methyl ~{N}-[4-[1-[(1~{R})-1-[5-[5-chloranyl-2-(1,2,3,4-tetrazol-1-yl)phenyl]-1-oxidanyl-pyridin-2-yl]-2-cyclopropyl-ethyl]pyrazol-4-yl]phenyl]carbamate 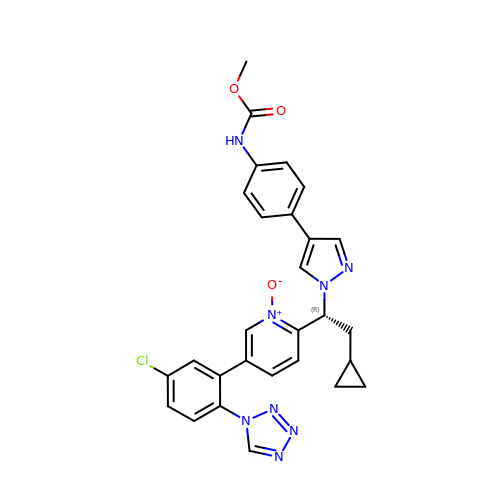| C28 H25 Cl N8 O3 | HRJWNRPDBZGIOP-HHHXNRCGSA-N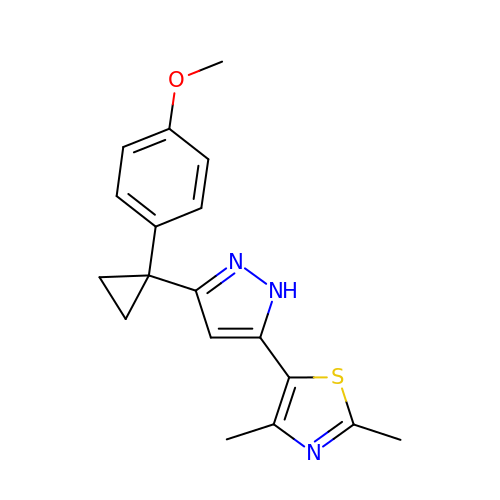5-{3-[1-(4-methoxyphenyl)cyclopropyl]-1H-pyrazol-5-yl}-2,4-dimethyl-1,3-thiazole | C18 H19 N3 O S | ONGUVGXZNLWDHM-UHFFFAOYSA-N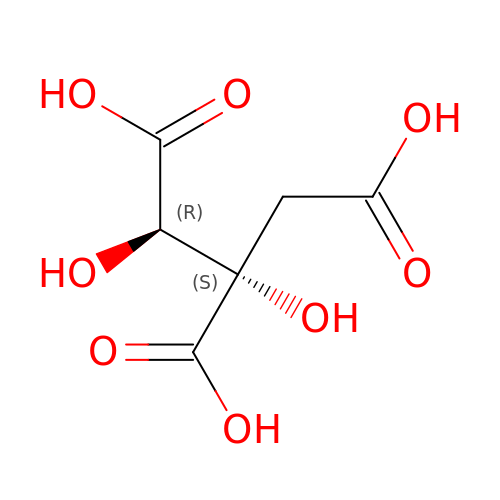3-C-carboxy-2-deoxy-L-threo-pentaric acid | C6 H8 O8 | ZMJBYMUCKBYSCP-DZSWIPIPSA-N> GSMASAAVANYEEEIVRPVADFSPSLWGDQFLSFSIKNQVAEKYAKEIEALKEQTRNMLLATGMKLADTLNLIDTIERLGISYHFEKEIDDILDQIYNQNSNCNDLCTSALQFRLLRQHGFNISPEIFSKFQDENGKFKESLASD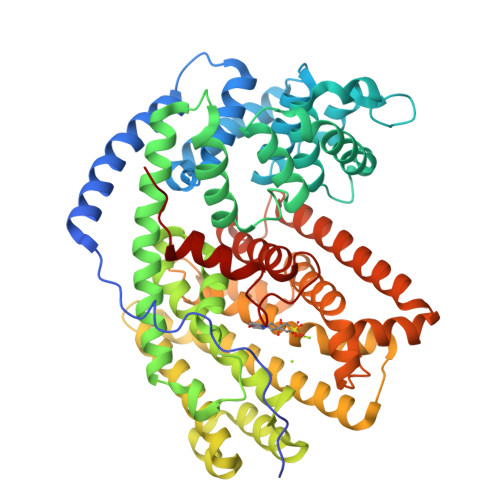VLGLLNLYEASHVRTHADDILEDALAFSTIHLESAAPHLKSPLREQVTHALEQCLHKGVPRVETRFFISSIYDKEQSKNNVLLRFAKLDFNLLQMLHKQELAQVSRWWKDLDFVTTLPYARDRVVECYFWALGVYFEPQYSQARVMLVKTISMISIVDDTFDAYGTVKELEAYTDAIQRWDINEIDRLPDYMKISYKAILDLYKDYEKELSSAGRSHIVCHAIERMKEVVRNYNVESTWFIEGYTPPVSEYLSNALATTTYYYLATTSYLGMKSATEQDFEWLSKNPKILEASVIICRVIDDTATYEVEKSRGQIATGIECCMRDYGISTKEAMAKFQNMAETAWKDINEGLLRPTPVSTEFLTPILNLARIVEVTYIHNLDGYTHPEKVLKPHIINLLVDSIKI> MIYMTFGEILKKERVSWKLSVKELSTLSGVSQTYISKLENGKRNFPSLETIFNLLIGFKTHIEYKMGSESPFYEINNSYLDEILIMFINSSNSTISDRDPNELITQFNEYYDVTIKKKQNENSKIESDIFSNKIKLVKGTTKKEVIEKPYFDLNWLLTQNEYEVFFDRSFLLDNNFLNKKHFTEKDMYYYNVLNDNDLKTIKDEIVVFLLNKYNYIKNKDDFFNIFTNSEDDKTKRDALYKILYETD;> GAMDPMVTKEFLKIKLECSDMYAQKLIDEAQGDENKLYDLFIQKLAERHTRPAIVEY

Normally, these elements reside passively integrated in host bacterial chromosomes under the control of a master repressor protein, Stl (SaPI transcription leftward). Instead, SaPI activation depends on the formation of a complex between Stl and specific phage proteins, which act as inducers of the SaPI life cycle. Contrary to the classical phage and SaPI repressors, which are dimers, the SaPI1 repressor StlSaPI1 presents a unique tetrameric conformation never seen before. To derepress SaPI1, the phage-encoded protein Sri binds to and induces a conformational change in the DNA binding domains of StlSaPI1, preventing the binding of the repressor to its cognate StlSaPI1 sites.

Our previous structural analysis suggested the importance of residue L201 for tetramerization since their mutual interaction projecting from the middle of α8 nucleates the hydrophobic core. In support of this, a StlSaPI1 repressor carrying an L201E mutation (StlSaPI1 L201E), which introduces a charged residue into this hydrophobic environment, formed dimers in solution and confirmed the role of this helix in StlSaPI1 tetramerization. Furthermore, we solved the structure of the Sri-StlSaPI1 L201E complex, confirming both the dimerization state of the L201E mutant and its ability to interact with Sri, as our previous co-expression and SEC-MALS experiments suggested. The Sri-StlSaPI1 L201E structure was determined at 2.97 Å resolution by molecular replacement using the wt Sri-StlSaPI1 monomer structure that was previously determined as a model. The asymmetric unit of the crystal showed a monomer of StlSaPI1 L201E bound to a molecule of Sri. This complex formed a dimer with the symmetric molecules with identical organisation to that observed for the dimer formed by subunits A and B in the crystal asymmetric unit of the wt Sri-StlSaPI1 complex (RMSD of 1.2 Å for the superimposition of 489 Cα atoms of wt dimer with mutant crystallographic dimer), confirming the A–B subunit organization for the dimeric StlSaPI1. The Sri molecule binds to StlSaPI1 L201E in a disposition identical to that previously observed in the wt Sri-StlSaPI1 complex, indicating that the L201E mutation did not affect StlSaPI1 binding to Sri. However, although the Sri fold in both wt and mutant StlSaPI1 complexes is identical (RMSD of 1.5 Å for superimposition of 42 Cα atoms), the 7 C-terminal residues were not visible in the complex with the StlSaPI1 L201E mutant. Corroborating this, the Sri-StlSaPI1 L201E complex was unstable during the purification process and we observed Sri released from the complex during gel filtration chromatography. In contrast, the plasmid expressing the dimeric StlSaPI1 L201E repressor showed extremely high reporter expression even in the absence of prophage induction, confirming its inability to cause repression.>[2x]MHHHHHHHHENLYFQGSKEKFWKISTPPEAYWNREQEKLNRQYNPILSMLTNQTGEAGRLSNISHLNYCEPDLRVTSVVTGFNNLPDRFKDFLLYLRCRNYSLLIDQPDKCAKKPFLLLAIKSLTPHFARRQAIRESWGQESNAGNQTVVRVFLLGQTPPEDNHPDLSDMLKFESEKHQDILMWNYRDTFFNLSLKEVLFLRWVSTSCPDTEF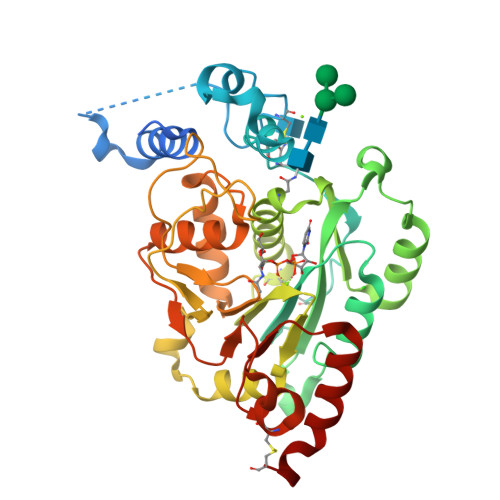VFKGDDDVFVNTHHILNYLNSLSKTKAKDLFIGDVIHNAGPHRDKKLKYYIPEVVYSGLYPPYAGGGGFLYSGHLALRLYHITDQVHLYPIDDVYTGMCLQKLGLVPEKHKGFRTFDIEEKNKNNICSYVDLMLVHSRKPQEMIDIWSQLQSAHLKC>VARPKSEDKKQALLEAATQAIAQ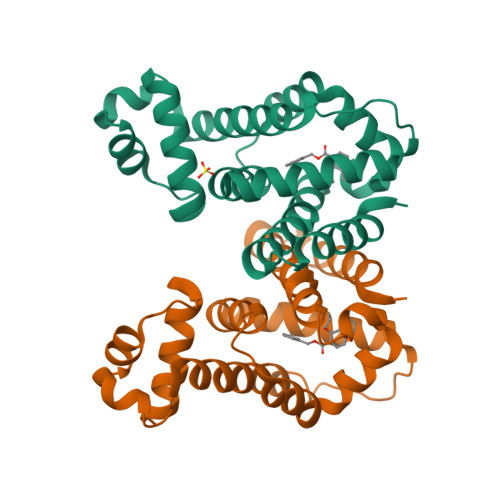SGIAASTAVIARNAGVAEGTLFRYFATKDELINTLYLHLRQDLWQSMIMELDRSITDAKMMTRFIWNSYISWGLNHPARHRAIRQLAVSEKLTKETEQRADDMFPELRDLAHRSVLMVFMSDEYRAFGDGLXLALAETTMDFAARDPARAGEYIALGFEAMWRALTREEQAAWSHPQFEK[4x]>[2x]MSASPPISAGDYLSAPEPDALKPAGPTPSQSRFQVDLVTESAGDGETTVGFDSSPPEYVAEPPPDGLRDSVSGGEKAKGRFRVVNFAASSPDAAPAETAQNGDTVMSEGSLHSSTGGQQHHHYDTHTNTYYLRTFGHNTIDAVPKIDFYRQTAAPLGEKLIRPTLSELHDELDKEPFEDGFANGEELTPAEESAAKDVSESKEPVRFGWVKGVMIRCMLNIWGVILYLRLPWITAQAGIVLTWIIILLSVTVTSITGLSISAISTNGKVKSGGTYFLISRSLGPELGGSIGLIFAFANAVGVAMHTVGFAATVRDLLQEYGAPIVDPINDIRIIGVVSVTVLLAISLAGMEWESKAQVLFFLVIMVSFANYLVGTLIPPSEDKASKGFFSYRADIFVQNLVPDWRGPDGTFFGMFSIFFPSATGILAGANISGDLKDPAIAIPKGTLMAIFWTTISYLAISATIGSCVVRDASGVLNDTVTPGWGACEGLACSYGWNFTECTQQHSCHYGLINYYQTMSMVSGFAPLITAGIFGATLSSALACLVSAAKVFQCLCEDQLYPLIGFFGKG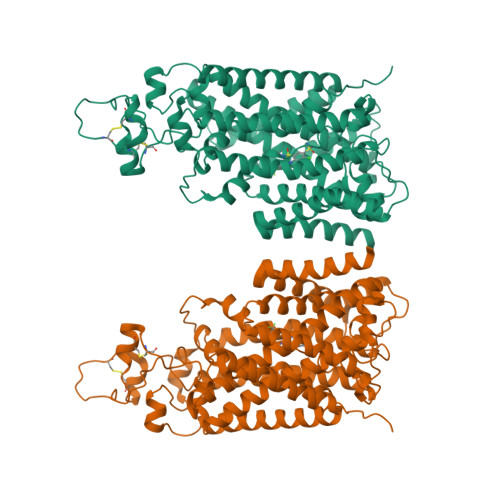YGKNKEPVRGYLLAYAIAVAFIIIAELNTIAPIISNFFLCSYALINFSCFHASITNSPGWRPSFQYYNKWAALFGAIISVVIMFLLTWWAALIAIGVVLFLLLYVIYKKPEVNWGSSVQAGSYNLALSYSVGLNEVEDHIKNYRPQCLVLTGPPNFRPALVDFVGTFTRNLSLMICGHVLIGPHKQRMPELQLIANGHTKWLNKRKIKAFYSDVIAEDLRRGVQILMQAAGLGRMKPNILVVGFKKNWQSAHPATVEDYIGILHDAFDFNYGVCVMRMREGLNVSKMMQAHINPVFDPAEDGKEASARVDPKALVKEEQATTIFQSEQGKKTIDIYWLFDDGGLTLLIPYLLGRKRRWSKCKIRVFVGGQINRMDQERKAIISLLSKFRLGFHEVHILPDINQNPRAEHTKRFEDMIAPFRLNDGFKDEATVNEMRRDCPWKISDEEITKNRVKSLRQVRLNEIVLDYSRDAALIVITLPIGRKGKCPSSLYMAWLETLSQDLRPPVILIRGNQENVLTFYCQ> GAACGACACTGACGGAGACTC;> CCGTCA;> TCGAGTCT;>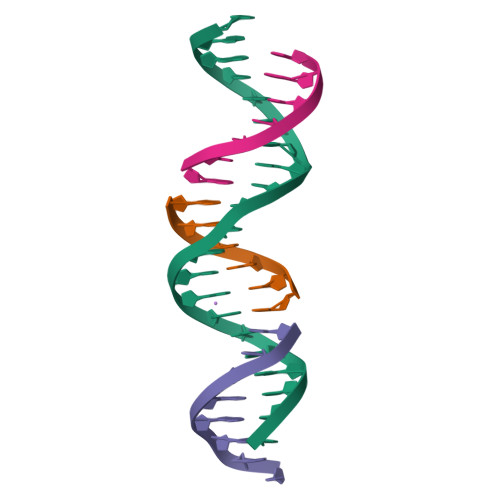 GTGTCGT2-[4-(diethylamino)-2-oxidanyl-phenyl]carbonylbenzoic 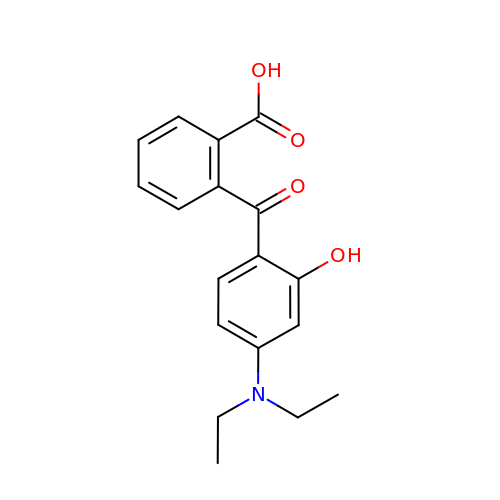acid | C18 H19 N O4 | FQNKTJPBXAZUGC-UHFFFAOYSA-N>GSHGGSMLTILKLGGSILSDKNVPYSIKWDNLERIAMEIKNALDYYKNQNKEIKLILVHGGGAFGHPVAKKYLKIEDGKKIFINM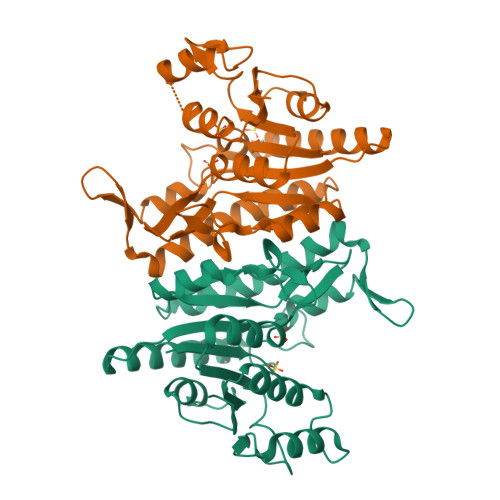EKGFWEIQRAMRRFNNIIIDTLQSYDIPAVSIQPSSFVVFGDKLIFDTSAIKEMLKRNLVPVIHGDIVIDDKNGYRIISGDDIVPYLANELKADLILYATDVDGVLIDNKPIKRIDKNNIYKILNYLSGSNSIDVTGGMKYKIEMIRKNKCRGFVFNGNKANNIYKALLGEVEGTEIDFSE[2x]>[3x]MDFLDFEKVFSFYSKATKKGFSPFFVPALEKAEEPAGNFFLDRKGNLFSIREDFTKTVLNHRKRYSPDSQIKVWYADFVYRYSGSDLVAEYQLGLEKVPRNSLDDSLEVLEIIVESASEFFEGPVIVEIGHTGVYEDLLKEIPKDLHEKVLNLIDTKNLAEIEFLSHMKKIDLSRVEKIIEDSIYRRSPEHLKTMDLPLSVREDLLSASSFLQEKFPTVSVEIDLTLARTIEEYCGLIFTIYDTSSS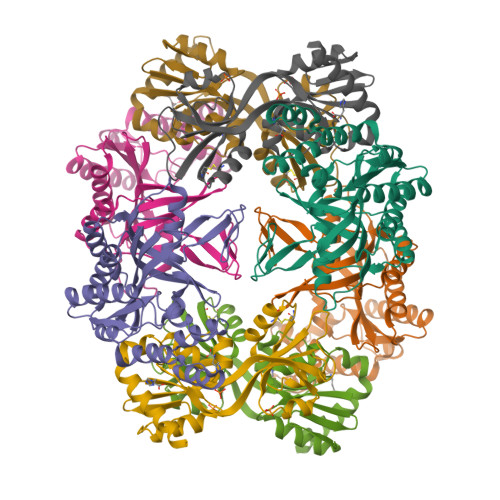RLVAAGGEYTVNGEKGVGGSIFLEGKTC;> MDFLDFEKVFSFYSKATKKGFSPFFVPALEKAEEPAGNFFLDRKGNLFSIREDFTKTVLNHRKRYSPESQIKVWYADFVYRYSGSDLVAEYQLGLEKVPRNSLDDSLEVLEIIVESASEFFEGPVIVEIGHTGLYEDLLKEIPKDLHEKVLNLIDTKNLAEIEFLSHMKKIDLSRVEKIIEDSIYRRSPEHLKTMDLPLSVREDLLSASSFLQEKFPTVSVEIDLTLARTIEEYCGLIFTIYDTSSSRLVAAGGEYTVNGEKGVGGSIFLEGKTC;>MLKLAIPKGRLEEKVMTYLKKTGVIFERESSILREGKDIVCFMVRPFDVPTYLVHGVADIGFCGTDVLLEKETSLIQPFFIPTNISRMVLAGPKGRGIPEGEKRIATKFPNVTQRYCESKGWHCRIIPLKGSVELAPIAGLSDLIVDITETGRTLKENNLEILDEIFVIRTHVVVNPVSYRTKREEVVSFLEKLQEVIEHDSNEQSRG[3x];> MLKLAIPKGRLEEKVMTYLKKTGVIFERESSILREGKDIVCFMVRPFDVPTYLVHGVADIGFCGTDVLLEKETSLIQPFFIPTNISRMVLAGPKGRGIPEGEKRIATKFPNVTQRYCESKGWHCRIIPLKGSVELAPIAGLSDLIVDITETGRTLKENNLEILDEIFVIRTHVVVNPVSYRTKREKVVSFLEKLQEVIEHDSNEQSRG> GUGUGCCCGGCAUGGGUGCAGUCUAUAGGGUGAGAGUCCCGAACUGUGAAGGCAGAAGUAACAGUUAGCCUAACGCAAGGGUGUCCGUGGCGACAUGGAAUCUGAAGGAAGCGGACGGCAAACCUUCGGUCUGAGGAACACGAACUUCAUAUGAGGCUAGGUAUCAAUGGAUGAGUUUGCAUAACAAAACAAAGUCCUUUCUGCCAAAGUUGGUACAGAGUAAAUGAAGCAGAUUGAUGAAGGGAAAGACUGCAUUCUUACCCGGGGAGGUCUGGAAACAGAAGUCAGCAGAAGUCAUAGUACCCUGUUCGCAGGGGAAGGACGGAACAAGUAUGGCGUUCGCGCCUAAGCUUGAACCGCCGUAUACCGAACGGUACGUACGGUGGUGUGG;> GUUAU

The self-splicing group II introns are bacterial and organellar ancestors of the nuclear spliceosome and retro-transposable elements of pharmacological and biotechnological importance. Besides catalyzing their self-splicing, group II introns also act as mobile retroelements, thus crucially contributing to genetic diversity throughout evolution. Integrating enzymatic, crystallographic, and simulation studies, we demonstrate how these introns recognize small molecules through their conserved active site. These RNA-binding small molecules selectively inhibit the two steps of splicing by adopting distinctive poses at different stages of catalysis, and by preventing crucial active site conformational changes that are essential for splicing progression.

We also determined a co-crystal structure at 3.1 Å resolution of Oi5eD1-5 and intronistat B in the state immediately following the first step of splicing, which is obtained in the presence of Mg2+ and K+. We had previously established, however, that immediately after 5’-exon hydrolysis these crystallization conditions trap the scissile phosphate in an unproductive conformation, which is unlikely to be of physiological relevance.> MSHHHHHHSGSGSGDKEIVEEVRKLVEEAKKRNEESNEEVKKLVEEAEEALKKAKGEEEVLKIAKEAFELAIEAAKRNLKVAKEAFELVIEAIKAITDDEAVLRLAELAAELAKSQLESLLKIAEAAMRLAASAIKAAKGDEAIVEIVRLLVEVAEEINKASNAVVKFLVEVAKEALKVAKGEEVVLEIARLAFELAIEAAKINLEVARLAFELVITAIEAITDDEAVLRLAKLAAELAKSQLESLLNIAEAAMELAASAIKAAKGDEAIVEIVRLLVEVAKEINKASNAVVEFLVE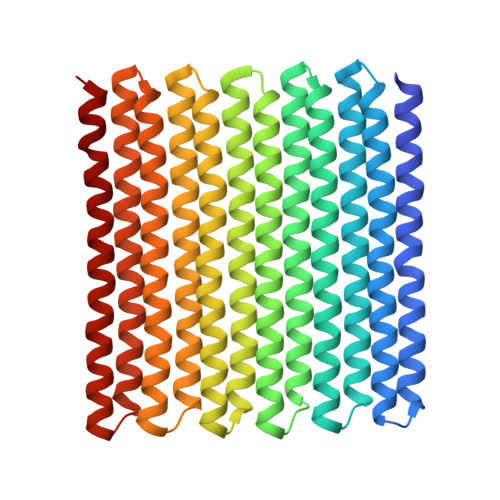VAEEALRVAKGEEVVLEIARLAFELAIEAARINLEVARLAFELVITAIEAITDDEAVLKLAELAAELAKSQLESLLRIAEAAMRLAASAIKAAKGDEAIVEIVRLLVEVAEEINKASNAVVEFLVEVAEEALRVAKGEEVVEEIAKLAKELADEAAKINEEVAKLAEELVKTAEEAITDDEARKKLRELAKKLRKSQEESKKRIKEAAEKLEASARKAAKG>[2x]QYVRIKNWGSGEILHDTLHHKATSDFTCKSKSCLGSIMNPKSLTRGPRDKPTPLEELLPHAIEFINQYYGSFKEAKIEEHL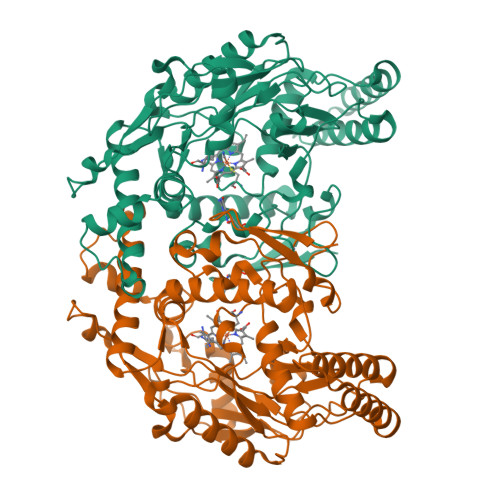ARLEAVTKEIETTGTYQLTLDELIFATKMAWRNAPRCIGRIQWSNLQVFDARNCSTAQEMFQHICRHILYATNNGNIRSAITVFPQRSDGKHDFRLWNSQLIRYAGYQMPDGTIRGDAATLEFTQLCIDLGWKPRYGRFDVLPLVLQADGQDPEVFEIPPDLVLEVTMEHPKYEWFQELGLKWYALPAVANMLLEVGGLEFPACPFNGWYMGTEIGVRDFCDTQRYNILEEVGRRMGLETHTLASLWKDRAVTEINVAVLHSFQKQNVTIMDHHTASESFMKHMQNEYRARGGCPADWIWLVPPVSGSITPVFHQEMLNYVLSPFYYYQIEPWKTHIW> MLEQPYLDLAKKVLDEGHFKPDRTHTGTYSIFGHQMRFDLSKGFPLLTTKKVPFGLIKSELLWFLHGDTNIRFLLQHRNHIWDEWAFEKWVKSDEYHGPDMTDFGHRSQKDPEFAAVYHEEMAKFDDRVLHDDAFAAKYGDLGLVYGSQWRAWHTSKGDTIDQLGDVIEQIKTHPYSRTLIVSAWNPEDVPTMALPPCHTLYQFYVNDGKLSLQLYQRSADIFLGVPFNIASYALLTHLVAHECGLEVGEFIHTFGDAHLYVNHLDQIKEQLSRTPRPAPTLQLNPDKHDI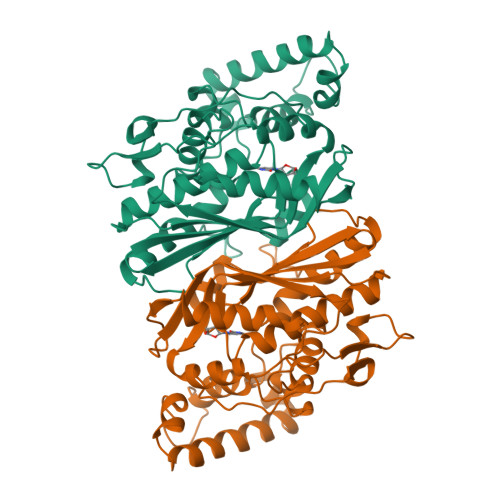FDFDMKDIKLLNYDPYPAIKAPVAV6-amino-2-{[2-(piperidin-1-yl)ethyl]amino}-3,5-dihydro-8H-imidazo[4,5-g]quinazolin-8-one 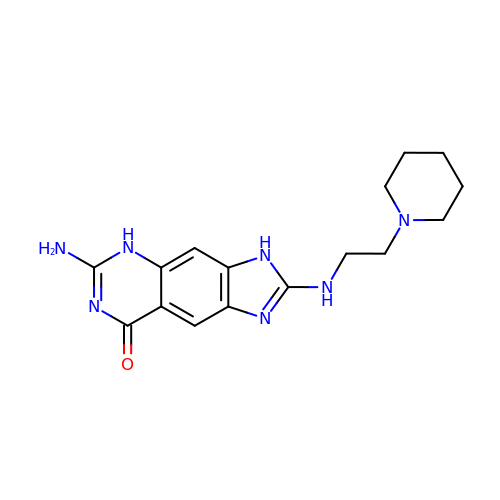| C16 H21 N7 O | BIGVTSCIEIRKFZ-UHFFFAOYSA-N>[2x]MASSSTAYYLKDAGFHIRNIPKAWNDWNLFH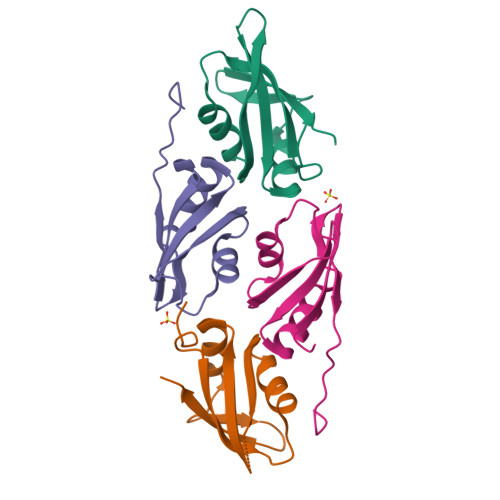VFQNFGKVSYCRVVGQSNDGQVQLGFVNMMSVADADEVRKNLNDGNLIGENFTLKVTDHKN;>[2x]DQENMLKISGYPGMLNTFGIAQLLTPYRVNGITITGAQSAVVALENKFQVYQAVQDFNGKKLDRNHKLQVSSLVVSSPAVPLE>MESLPVIAAPSMWTRPQIKDFKEKIQQDADSVITVGRGEVVTVRVPTHEEGSYLFWEFATDNYDIGFGVYFEWTDSPNTAVSVHVSESSDDDEEEEENIGCEEKAKKNANKPLLDEIVPVYRRDCHEEVYAGSHQYPGRGVYLLKFDNSYSLWRSKSVYYRVYYTR[2x];>[2x]GAMGPVYKDLEIDVCNTPPPECINDLLKSVDSEEIREYCKKKKWIIPEIPTNIERAMNQ

ACBD3 is a Golgi resident protein involved in the maintenance of the Golgi structure and regulation of intracellular trafficking between the endoplasmic reticulum and the Golgi. However, in enterovirus-infected cells, the ACBD3 GOLD domain interacts preferentially with viral non-structural 3A proteins, which causes re-localization of ACBD3 to the sites of virus replication. In this study, we present a structural, biochemical, and biological characterization of the complexes composed of human ACBD3 and the 3A proteins of four representative enteroviruses. The crystal structures revealed the details of the ACBD3-3A interaction, the 3A-3A interaction causing the assembly of the ACBD3-3A heterotetramers, the interaction between the ACBD3-3A complex and the lipid bilayer, and the roles of these interactions in facilitation of enterovirus replication.

Of the six GOLD: enterovirus 3A complexes, only GOLD: 3A/EVD68 and GOLD: 3A/RVB14 formed crystals that diffracted to a resolution suitable for subsequent structure determination (i.e. 2.3 Å and 2.9 Å, respectively). Analysis of the crystal structures of the GOLD: 3A complexes revealed that the 3A proteins formed either one of the crystal-packing contacts (as in the case of EVD68 and PV1) or contacts with the second 3A molecule when two GOLD: 3A complexes per asymmetric unit were present (as in the case of EVA71 and RVB14). This putative dimerization interface is formed by the two central alpha helices of the 3A proteins, which are bent 180° to form a helical hairpin. Surprisingly, the C termini of the 3A proteins, which in the cellular environment are anchored to the membranes, are located on the opposite sides of the GOLD: 3A heterotetramers. The dissociation constants of the GOLD: enterovirus 3A complexes ranged approximately from 1 μM (EVD68 and RVB14) to 15 μM (EVA71). The overall structures of all solved GOLD: 3A complexes are highly similar to each other.>GLIVDTRDVEERVHVMRKTKLAPTVAHGVFNPEFGPAALSNKDPRLNEGVVLDEVIFSKHKGDTKMSAEDKALFRRCAADYASRLHSVLGTANAPLSIYEAIKGVDGLDAMEPDTAPGLPWALQGKRRGALIDFENGTVGPEVEAALKLMEKREYKFACQTFLKDEIRPMEKVRAGKTRIVDVLPVEHILYTRMMIGRFCAQMHSNNGPQIGSAVGCNPDVDWQRFGTHFAQYRNVWDVDYSAFDANHCSDAMNIMFEEVFRTEFGFHPNAEWILKTLVNTEHAYENKRITVEGGMPSGCSATSIINTILNNIYVLYALRRHYEGVELDTYTMISYGDDIVVASDYDLDFEALKPHFKSLGQTITPADKSDKGFVLGHSITDVTFLKRHFHMDYGTGFYKPVMASKTLEAILSFARRGTIQEKLISVAGLAVHSGPDEYRRLFEPFQGLFEIPSYRSLYLRWVNAVCGDAAAAKEHHHHHH[2x];> GPYAGPLERQRPLKVRAKLPRQE

The core enzyme in the replication machinery is the viral RNA-dependent RNA polymerase (RdRP) 3Dpol. The enzyme adopts the canonical closed right-hand polymerase fold, consisting of fingers, palm, and thumb subdomains that encircles seven conserved structural motifs (A to G), playing critical roles in rNTP substrate recognition, template/primer binding and catalysis. 3Dpol uses 3B as a primer protein to initiate the replication process. Unlike other picornaviruses, the animal pathogen foot-and-mouth disease virus (FMDV), encodes three non-identical copies of the 3B (3B1, 3B2, and 3B3) that could be specialized in different functions within the replication complex.

The best diffracting crystals were those of the 3DpolHis-3B1 complex grown in the presence of UTP and Mn2+. These crystals, orthorhombic P212121, contained two 3Dpol molecules in the asymmetric unit and diffracted at 1.7 Å resolution. The quality of the electron density for the 3B1 molecule in the P212121 crystals allowed to interpret with confidence the 3B1 amino acids from G5 to R21. In the structure of the 3DpolHis-3B1 complex, 3B1 molecule binds the bottom of the palms of two confronted 3Dpol molecules (named 3DpolI and 3DpolII), in an almost equivalent way. The 3B1 binding region in both molecules consists in a hydrophobic cavity formed by residues: from H322 to V326, T330 and from Y346 to L348. These cavities are occupied by two hydrophobic residues (G5 and P6; region I) and (L19 and P20, region II) located at the N- and C-terminus of 3B1, respectively. In region I these interactions involve the main and side chains of the 3B1 residue R9 and the main chain oxygens of residues R320 and E324 in 3DpolI. In region II, an equivalent interaction is established between the 3Dpol II main chain residues H322 and E324 and the main and side chains of R16 in 3B1. Region II also shows an additional polar contact involving the side chain of residue R21 in 3B1 and the main chain carboxyl oxygen of D345 in 3Dpol, slightly increasing the interaction surface (508.2Å) at this binding site. Furthermore, the two 3Dpol molecules linked by 3B1, interact with each other through contacts mediated by residues from G125 to P141 in the fingers sub-domain, forming long fibers along a diagonal in the ab plane in the crystal packing.Hypusine (N-(4-amino-2-hydroxybutyl) lysine), an unusual amino acid, is formed by the post-translational modification of a lysine residue with the addition of the aminobutyl moiety from the polyamine spermidine. The hypusine modification of eIF5A is catalyzed by deoxyhypusine synthase (DHS), followed by the hydroxylation of deoxyhypusine by deoxyhypusine hydroxylase (DOHH). DHS catalyzes a NAD+-dependent reaction that synthesizes deoxyhypusine (N-(4-aminobutyl) lysine) by transferring the butylamine moiety of spermidine to a specific lysine residue of eIF5A. Consistent with archaea sharing a requirement for hypusine for the function of translation factor aIF5A, both the modification and DHS gene homologues have been identified.

In this study, we determined the crystal structure of DHS from Pyrococcus horikoshii OT3 (PhoDHS), with NAD+-bound, at 2.2 Å resolution. Similar to DHS from other organisms, this tetramer is a dimer of dimers with a point group of D2, generated by two local 2-fold axes that are perpendicular to each other. Interestingly, unlike human and T. brucei DHS, PhoDHS contains only two bound NAD+ molecules and shows a difference in the NAD+-bound and NAD+-free monomeric conformations. Two bulky electron density blocks shaped as NAD+ were distinguished at the interface between molA and molD of the PhoDHS tetramer after several cycles of refinement and were later assigned as NAD+. Those NAD+ molecules were naturally captured during the expression of the enzyme in Escherichia coli, since no NAD+ was added during purification and crystallization processes. The two NAD+ molecules (NAD1 and NAD2) are embraced individually by molA and molD of PhoDHS in a sandwich binding manner and insert their ends into the pockets of molA, and molD with 2-fold symmetry. Bound NAD+ is proximal to a loop (V288–P299 (hereafter named “the binding loop”)) that displays very different conformations in each monomer of the PhoDHS tetramer. Notably, in molA and molD, observed to bind NAD+, the binding loop adopts two different conformations (right): in molA, the binding loop positions away from NAD+ (conf), while in molD, the binding loop adopts another conformation to access NAD+ (conf). In the molB and molC of the PhoDHS tetramer, where NAD+ is absent, the binding loop is disordered or only partially visible. Strikingly, our structure presents a simultaneous combination of three different conformations at the spermidine binding site that are reflective of a three-state conformational regulation of DHS by NAD+: the apo form, the open form, and the closed/reaction form.

>[4x]MKAKDIVLKKSEKIEGVEVKGPWLDDAQSLEEVVSYYYRIGFQATHLGRAIEIWRKVEEKRERGEEIRVFLGYTSNIISSGLREIIAWLVKEKKVDVIVTTAGGVEEDFIKSLKPFILGDWEVDDAELRKKGVNRIGNIFVPNDRYIEFEKYMIPFFERVLKIEEKLSRPLTASEFIYEMGRYMDEKLGKEKEKSVIYWAYKNNIPIFCPAITDGSIGDMLYFFKEERRDSRLIIDIANDIVKLNNLAITAKETASIILGGSLPKHAIINANLFRGGTDYAIYISTAVPWDGSLSGAPPREGVSWGKIKAKADYVEVWGDATLIFPILVWMVMKARGQGYAQ>MGSSHHHHHHSQDPNSATANGSSKGSFEVPKVEVRFTKLFIDGKFVDAVSGKTFETRDPRTGEVIASIAEGDKADVDLAVKAAREAFDNGPWPRMTGYERGRILHRFADLIDEHVEELAALDTVDAGKLFAVGKARDIPGAAHLLRYYAGAADKVHGATLKMAQRMHGYTLKEPVGVVGHIVPWNYPTTMFFFKVGPALAAGCAVVVKPAEQTPLSALFYAHLAREAGVPAGVLNVVPGFGPTAGAAVAAHMDVDKVSFTGSTEVGRLVMRAAAESNLKPVSLELGGK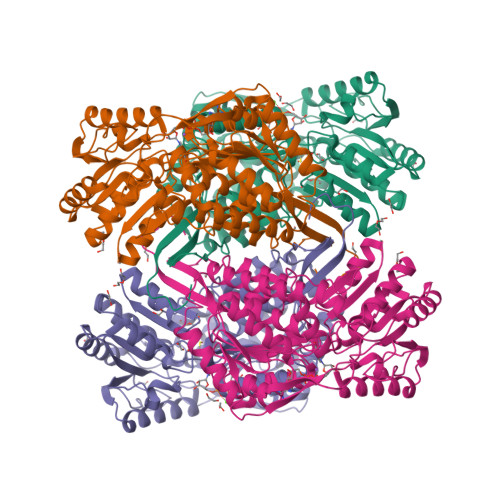SPVIVFDDADLDMAVNLVNFATYTNKGEICVAGTRIYVQEGIYDEFVKKAAELASKSVVGDPFNPSVSQGPQVDKDQYEKVLRYIDIGKREGATLVTGGKPCGDKGYYIEPTIFTDVKDDMTIAQDEIFGPVMALMKFKTVEEVIQKANNTRYGLAAGIVTKNIDVANTVSRSIRAGAIWINCYFAFDPDAPFGGYKMSGFGKDMGMDALDKYLQTKTVVTPLYNTPWL[2x]5-chloranyl-4-imidazo[1,2-a]pyridin-3-yl-N-(3-methyl-1-piperidin-4-yl-pyrazol-4-yl)pyrimidin-2-amine | C20 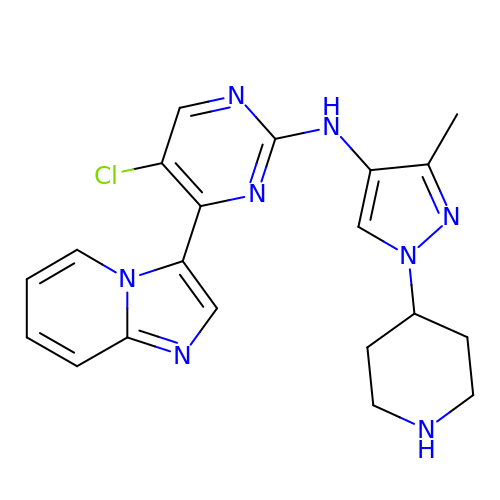H21 Cl N8 | JVFLXTNKVBOVBS-UHFFFAOYSA-N> SHMPASVQLHTAVEMHHWCIPFSVDGQPAPSLRWLFNGSVLNETSFIFTEFLEP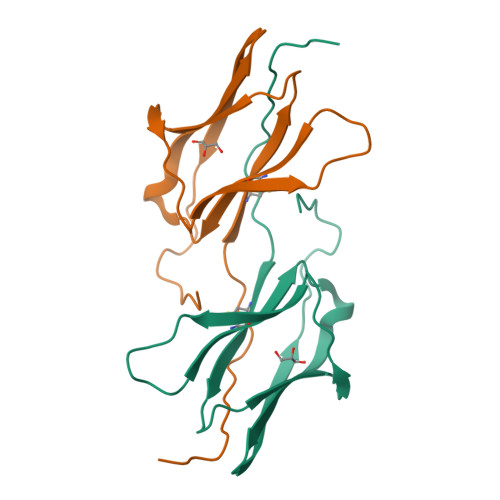AANETVRHGCLRLNQPTHVNNGNYTLLAANPFGQASASIMAAFMDNPFEFNPEDPIPDTNSTSGDPVEKKDE Human short coiled coil protein (SCOC) is an effector of the Golgi resident GTPase Arl1 and was recently identified as a positive regulator of autophagy in a genome-wide siRNA screen. SCOC interacts with fasciculation and elongation protein zeta 1 (FEZ1). At least four different human SCOC isoforms are known. Their N-termini are variable, whereas the approx. 70 residues long coiled coil domain is highly conserved, also among different species, highlighting its functional importance. SCOC is a dimeric coiled coil protein with an unusual high incidence of polar and charged residues at half of the heptad a-positions.

We determined the crystal structure of the coiled coil domain of human SCOC isoform 1 at 2.7 Å resolution. The structure was solved by single wavelength anomalous diffraction (SAD) phasing using selenomethionine labeled crystals of the L105M SCOC mutant. The final model comprises residues 86-147. SCOC is a parallel left-handed coiled coil homodimer. The structure contains eight heptad repeats and has a length of about 80 Å. The asymmetric unit contains three SCOC molecules. Molecules A and B form dimer AB and the second dimer CC’ is composed of molecule C and a symmetry related copy of C. Dimer CC’ is a regular coiled coil, whereas chains A and B are not as tightly packed because molecule A is bent with a bulge around residues A116. The coiled coil pitch of dimer AB (residues 97-143) is 129 Å and 151 Å for dimer CC’ as calculated with the program TWISTER. Remarkably, half of the a heptad positions at the core of the coiled coil are occupied by polar and charged residues. Instead, we explain this plasticity with the enrichment of polar and charged residues at the a/d-heptad positions.

>MMNADMDAVDAENQVELEEKTRLINQVMELQHTLEDLSARVDAVKEENLKLKSENQVLGQYIENLMSASSVFQTTDTKSKRK[3x]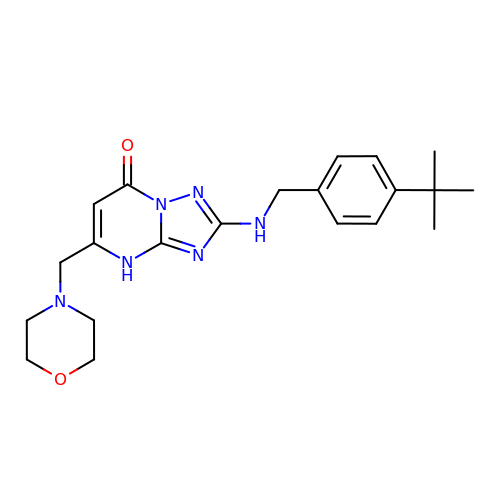(8R)-2-{[(4-tert-butylphenyl)methyl]amino}-5-[(morpholin-4-yl)methyl][1,2,4]triazolo[1,5-a]pyrimidin-7(4H)-one | C21 H28 N6 O2 | RPOXTKKWAOVEIJ-UHFFFAOYSA-N>[2x]MKIAVLGATGRAGSAIVAEARRRGHEVLAVVRDPQKAADR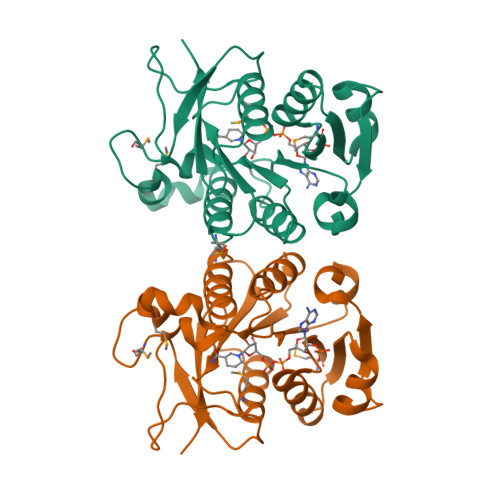LGATVATLVKEPLVLTEADLDSVDAVVDALSVPWGSGRGYLHLDFATHLVSLLRNSDTLAVFILGSASLAMPGADHPMILDFPESAASQPWYDGALYQYYEYQFLQMNANVNWIGISPSEAFPSGPATSYVAGKDTLLVGEDGQSHITTGNMALAILDQLEHPTAIRDRIVVRDADLEHHHHHH>MGRKKIQITRIMDERNRQVTFTKRKFGLMKKAYELSVLC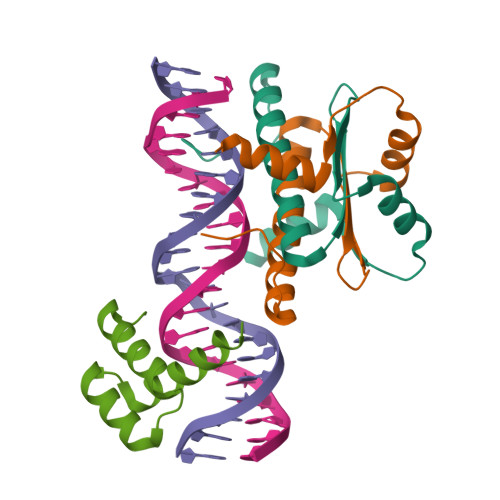DCEIALIIFNSSNKLFQYASTDMDKVLLKYTEYSEPHESRTNTDILETLKRREHRG[6x];>[3x]RRRKPRVLFSQAQVYELERRFKQQRYLSAPERDQLASVLKLTSTQVKIWFQNRRYKSKRQR(5R,7S,10S)-10-tert-butyl-N-{(1R,2R)-1-[(cyclopropylsulfonyl)carbamoyl]-2-ethylcyclopropyl}-15,15-dimethyl-3,9,12-trioxo-6,7,9,10,11,12,14,15,16,17,18,19-dodecahydro-1H,5H-2,23:5,8-dimethano-4,13,2,8,11-benzodioxatriazacyclohenicosine-7(3H)-carboxamide 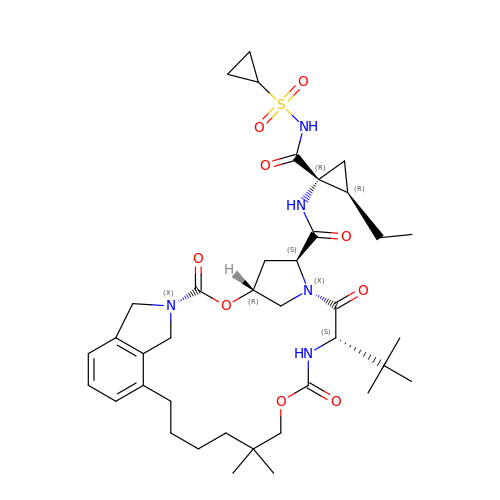| C38 H55 N5 O9 S | KUQWGLQLLVFLSM-ONAXAZCASA-N> SLSDKDKAAVRALWSKIGKSSDAIGNDALSRMIVVYPQTKIYFSHWPDVTPGSPNIKAHGKKVMGGIALAVSKIDDLKTGLMELSEQHAYKLRVDPSNFKIL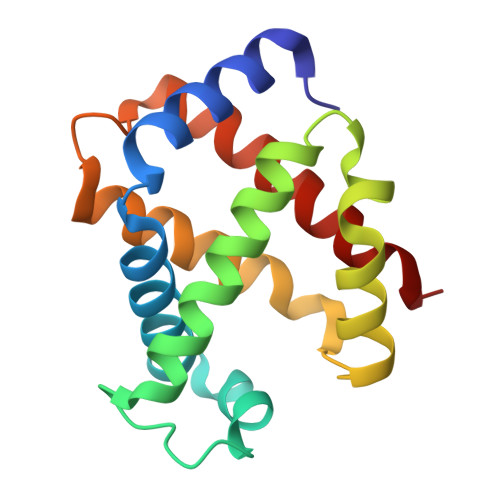NHCILVVISTMFPKEFTPEAHVSLDKFLSGVALALAERYR> AHHHHHHPGGPGSENLYFQGGSSGTQDVVYFPPKILTSVGSNASFHCIYKNENQIISSKQIVWWR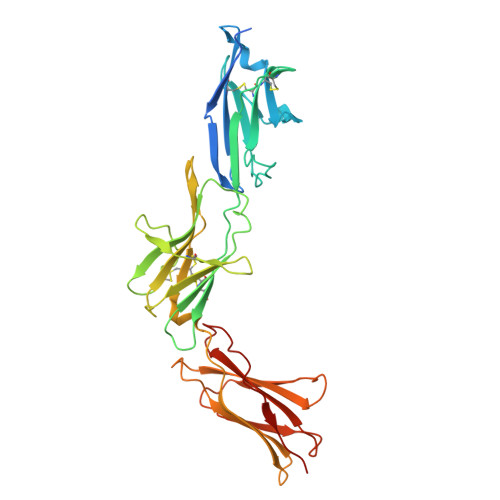NLAEKIPEIQYSIVSDRVSKVTFSNLKATRPRGKFTYDAVYCCNEQACHHRYAELYVIDVNINISCETDGYLTKMTCRWSPSTIQSLVGSTVQLRYHRRSLYCPDSPSIHPTSEPKNCVLQRDGFYECVFQPIFLLSGYTMWIRINHSLGSLDSPPTCVLPDSVVKPLPPSNVKAEITVNTGLLKVSWEKPVFPENNLQFQIRYGLSGKEIQWKTHEVFDAKSKSASLLVSDLSAVYVVQVRCRRLDGLGYWSNWSSPAYTLVMD>MQTVVKASYWFPASEFPVTDIDSSLFTHLFCAFADLNSQTNQVTVSSANQPKFSTFTQTVQRRNPSVKTLLSIGGGIADKTAYASMASNPTSRKSFIDSSIRVARSYGFHGLDLDWEYPSSATEMTNFGTLLREWRSAVVAEASSSGKPRLLLAAAVFYSNNYYSVLYPVSAVASSLDWVNLMAYDFYGPGWSRVTGPPAALFDPSNAGPSGDAGTRSWIQAGLPAKKAVLGFPYYGYAWRLTNANSHSYYAPTTGAAISPDGSIGYGQIRKFIVDNGATTVYNSTVVGDYCYAGTNWIGYDDNQSIVTKVR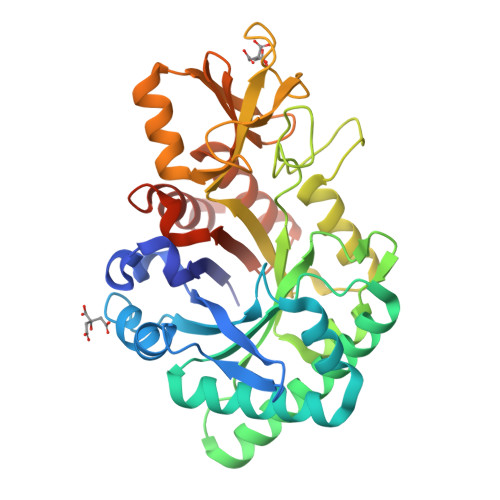YAKQRGLLGYFSWHVGADDNSGLSRAASQAWDATTATTRTIQKV[4x]ISOCITRIC ACID | C6 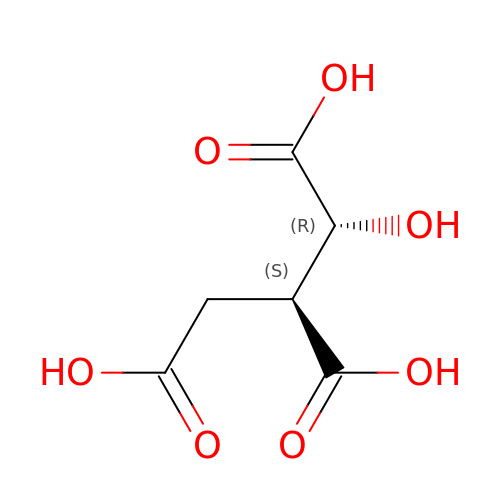H8 O7 | ODBLHEXUDAPZAU-ZAFYKAAXSA-N> MRSVLRKAGSPRKARRARLNPLVLLLDAALTGELEVVQQAVKEMNDPSQPNEEGITALHNAICGANYSIVDFLITAGANVNSPDSHGWTPLHCAASCNDTVICMALVQHGAAIFATTLSDGATAFEKCDPYREGYADCATYLADVEQSMGLMNSGAVY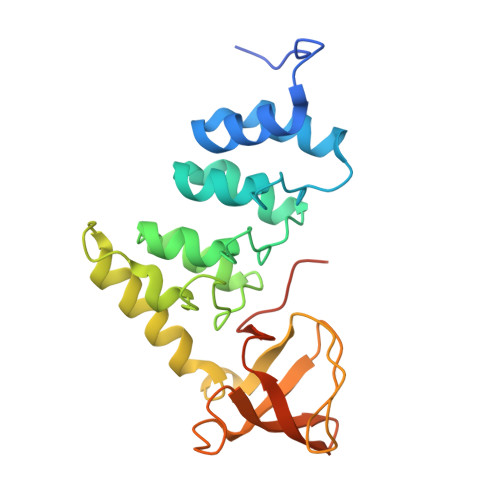ALWDYSAEFGDELSFREGESVTVLRRDGPEETDWWWAALHGQEGYVPRNYFGLFPRVKPQRSKVKHHHHHH>ASHHHHHHMPCEELDIVWNNIKAEARALADCEPMLASFYHATLLKHENLGSALSYMLANKLASPIMPAIAIREVVEEAYAADPEMIASAACDIQAVRTRDPAVDKYSTPL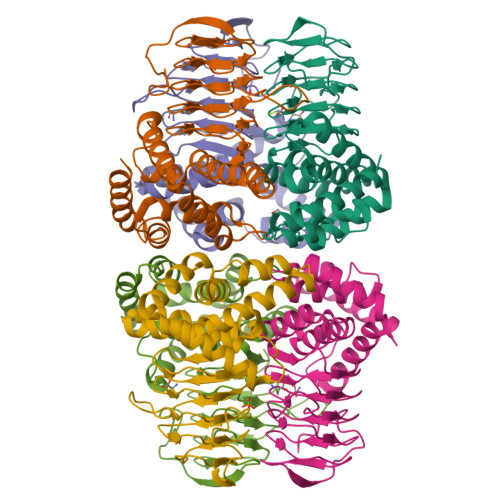LYLKGFHALQAYRIGHWLWTQGRRALAIFLQNQVSVSFQVDIHPAAKIGRGIMLDHATGIVVGETAVIEDDVSILQSVTLGGTGKTSGDRHPKIREGVMIGAGAKILGNIEVGRGAKIGAGSVVLQPVPPHTTAAGVPARIVGKPESDKPAMDMDQHFNGIHHTFEYGDGI[6x]>GLEAKKEENLADWYSQVITKSEMIEYHDISGCYILRPWAYAIWEAIKDFFDAEIKKLGVENCYFPMFVSQSALEKEKTHVADFAPEVAWVTRSGKTELAEPIAIRPTSETVMYPAYAKWVQSHRDLPIKLNQWCNVVRWEFKHPQPFLRTREFLWQEGHSAFATMEEAAEEVLQILDLYAQVYEELLAIPVVKGRKTEKEKFAGGDYTTTIEAFISASGRAIQGGTSHHLGQNFSKMFEIVFEDPKIPGEKQFAYQNSWGLTTRTIGVMTMVHGDNMGLVLPPRVACVQVVIIPCGITNALSEEDKEALIAKCNDYRRRLLSVNIRVRADLRDNYSPGWKFNHWELKGVPIRLEVGPRDMKSCQFVAVRRDTGEKLTVAENEAETKLQAILEDIQVTLFTRASEDLKTHMVVANTMEDFQKILDSGKIVQIPFCGEIDCEDWIKKTTARDQDLEPGAPSMGAKSLCIPFKPLCELQPGAKCVCGKNPAKYYTLFGRSY[2x]

PARS1 is one of the aminoacyl‐tRNA synthetases (ARSs), which mediate the covalent ligation of amino acids to their cognate tRNAs for protein synthesis (Kim et al, 2011; Kwon et al, 2019). PARS1 catalyzes the covalent linkage of proline to tRNAPro. Unlike the other ARSs, PARS1 exists as a part of the bifunctional enzyme, glutamyl‐prolyl‐tRNA synthetase 1 (EPRS1), which comprises glutamyl‐tRNA synthetase 1 (EARS1), three repeats of WHEP domain, and PARS1 (Kwon et al, 2019). PARS1 is a homodimer formed by the PARS1 protomers A and B (Zhou et al, 2013).

The piperidine ring moiety of DWN compounds occupies a proline‐binding site and a ketone group (DWN11251, DWN11748, and DWN11761) or alkane group (DWN12088) connects the piperidine ring with the bicyclic ring, similar to HF (Son et al, 2013). DWN12088 and DWN11251 bound to PARS1 protomers asymmetrically (compounds with asymmetric binding, ABC), whereas HF, DWN11748, and DWN11761 bound symmetrically (compounds with symmetric binding, SBC). More specifically, protomers A and B of SBC‐bound PARS1 and protomer A of ABC‐bound PARS1 showed similar structures to each other, whereas protomer B of ABC‐bound PARS1 was different from the others in terms of the binding of both ATP and the compounds. The most striking difference between the structures was the loss of the electron density map of ATP in protomer B of the DWN12088‐bound structure. However, in protomer B complexed with DWN12088, there was no hydrogen bond due to the absence of an ATP molecule. In contrast, protomer A made over 10 more hydrogen bonds than protomer B in the complexes with ABC, implying the flexible or weakened binding of ATP in PARS1 protomer B. While the ketone group of the SBC formed stable hydrogen bonds with ATP, contributing to their tight binding to PARS1, DWN12088 did not have a ketone group in the bridge, which could decrease the rigidity of bicyclic ring orientation. In fact, the electron density of the bicyclic ring moiety of DWN12088 in protomer B of the complex structure was not well defined, and the R‐loop interacting with the bicyclic ring moiety was almost disordered, implying a potential loose binding of DWN12088 in PARS1 protomer B. On the other hand, when the first DWN12088 molecule binds to PARS1 protomer A, the second DWN12088 molecule could not bind tightly to protomer B due to allosteric effects. This negative cooperativity would make it difficult to inhibit the prolylation activity of PARS1 protomer B, broadening dose–response curve.>[2x]MAFDTYIKLDKVDGESTDDKHKKWIEVLGFAWGAGNECTMESGTQGLNTGKAMMSVLRVTKWMDCASVKLASAAVQGQNFPTLELEICTQAGDKFAFCIYKFTHVAVSSYQCSGATGGSD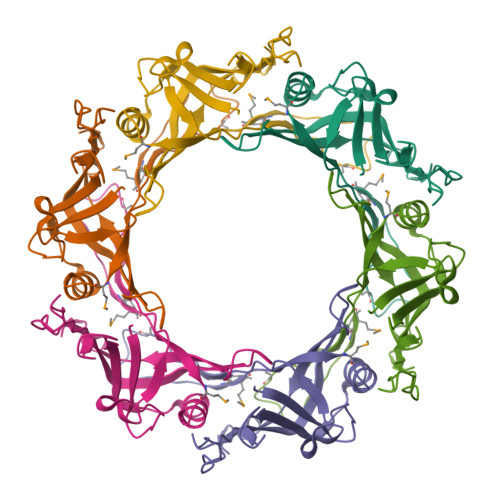RPQETIDFAYKEVTWEYVPQDQNGKAGGKIGPEGWSLITNKKK[(2S)-2-hydroxy-3-(1H-1,2,4-triazol-1-yl)propyl]phosphonic acid | C5 H10 N3 O4 P | 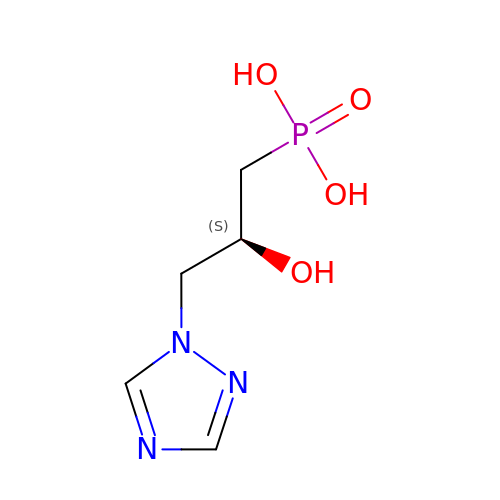ZXKJPBBOMRHTCH-YFKPBYRVSA-N Chalcone synthase (CHS) and chalcone isomerase (CHI) catalyze the first two committed steps of the flavonoid pathway that plays a pivotal role in the growth and reproduction of land plants, including UV protection, pigmentation, symbiotic nitrogen fixation, and pathogen resistance. Based on the obtained X-ray crystal structures of CHS, CHI, and chalcone isomerase-like protein (CHIL) from the same monocotyledon, Panicum virgatum, along with the results of the steady-state kinetics, spectroscopic/thermodynamic analyses, intermolecular interactions, and their effect on each catalytic step are proposed. The production of these value-added products also offers the prospect of increasing the value of the crop, especially because many of these compounds are soluble and readily extracted. This study characterized the enzymes involved in the first two committed steps of the flavonoid pathway, CHS and CHI, and the non-catalytic protein CHIL. Through crystal structure, molecular docking, mutagenesis, kinetic analyses, ITC, and FRET analysis, our study provides evidence supporting a revised catalytic reaction mechanism for monocot CHS and CHI and identified an intermolecular interaction of CHS with both CHI and CHIL in a non-competitive manner.

The asymmetric unit contained two molecules of PvCHI that did not display any significant interaction between them. As predicted, PDBePISA calculated that interaction between two PvCHI molecules in the asymmetric unit was low with a ΔiG of 1.1 kcal mol−1 and a CSS of 0.00, indicating its likely monomeric nature in solution. Among 237 residues in the native PvCHI, the electron density corresponding to the residues from 4 to 217 and 4 to 216 of the A and B molecules, respectively, were resolved, indicating the disordered nature of both N- and C- terminals. The three-dimensional structure of PvCHI displayed an open-faced β-sandwich fold with six anti-parallel β-sheets (β1–β6) and seven α-helices (α1–α7). The observed temperature factors for residues 35–39 and those constituting the α4 helix in PvCHI were elevated compared to other residues, indicating the intrinsic flexibility that allows the substrate to enter with a plausible induced fit. In addition, in the apo-form crystal structures of both PvCHI and SbCHI, the sidechain of Arg-35 in PvCHI (Arg-34 in SbCHI) was positioned at the substrate-entrance site and hydrogen bonded to both Thr-47 and Tyr-190 through water-molecules. The substrate specificity of type I and II CHIs has previously been attributed to the difference between Ser-190 and Ile-191 in type II vs. Thr and Met, respectively, in type I. PvCHI has Ser-190/Ile-191 in the α6 region and displayed significant activity toward isoliquiritigenin. The reaction rates for varying concentrations of naringenin chalcone displayed a typical Michaelis–Menten kinetics with a Vmax of 8012 μM s−1 and a Km of 16.04 μM.

>[2x]MAAVSEVAVDGVVFPPVARPPGSGRSHFLAGAGVRGMEIGGNFIKFTAIGVYLEEGAAVSALAKKWAGKSADELAADAAFFRDVVTGDFEKFTRVTMILPLTGEQYSGKVTENCVAYWKAVGVYTDAEGAAVDKFKEAFKPETFPPGASILFTHSPAGVLTVAFSKDSSVPESGGVAIDNKPLCEAVLESIIGEHGVSPAAKLSVAARVSELLKEASPAGGAPQAAAEPAVPVSAEF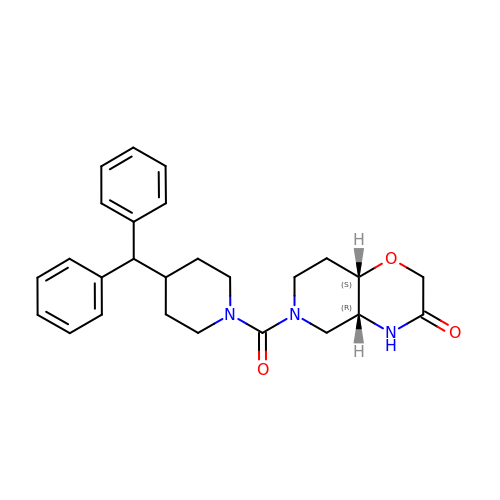(4aR,8aS)-6-[4-(diphenylmethyl)piperidin-1-yl]carbonyl-4,4a,5,7,8,8a-hexahydropyrido[4,3-b][1,4]oxazin-3-one | C26 H31 N3 O3 | ARSYSYCENXVYHJ-UHFFFAOYSA-N> MNLAQAFKENHSIRLGLTAKDWKEAVKLSVTPLIESGAVKPEYYNAIIESTESYGPYYILMPGMAMPHARPEAGVQRDAFSLVTLTEPVTFTDGKEVQVLLALAATSSKIHTSVAIPQIIALFEL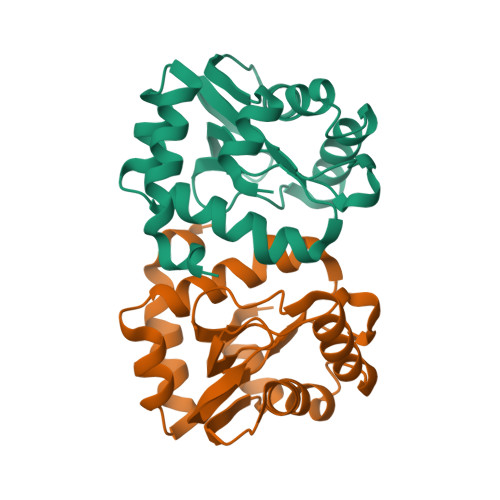DHSIERLVNCKTPEEVLAMVEESKSSPYLEGLDLDS> AHQ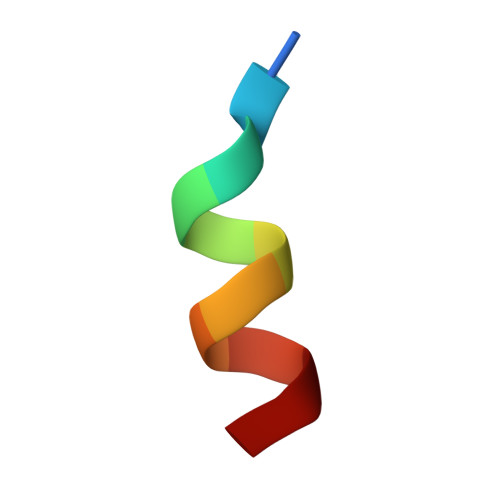LLRYLLDA> MIIFSGGTGTPKLLDGLKEILPEEELTVVVNTAEDLWVSGNLISPDLDTVLYLFSDQIDRKRWWGIENDTFGTYERMKELGIEEGLKLGDRDRATHIIRSNIIRDGASLTDSTVKLSSLFGIKANILPMSDDPVSTYIETAEGIMHFQDFWIGKRGEPDVRGVDIRGVSEASISPKVLEAFEKEENILIGPSNPITSIGPIISLPGMRELLKK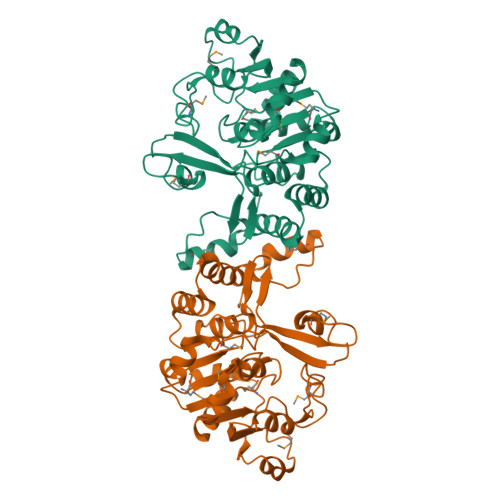KKVVAVSPIIGNAPVSGPAGKLMPACGIEVSSMGVAEYYQDFLDVFVFDERDRADEFAFERLGCHASRADTLMTSTEKSKELAEIVVQAFLEHHHHHH> EIMAVDIYVNPPRVDVFHGTPPAWSSFGNKTIWGGNEWVDDSPTRSDIEKRDKEITAYKNTLSAQQKENENKRTEAGKRLSAAIAAREKDENTLKTLRAGNADAADITRQEFRLLQAELREYGFRTEIAGYDALRLHTESRMLFADADSLRISPREARSLIEQAEKRQKDAQNADKKAADML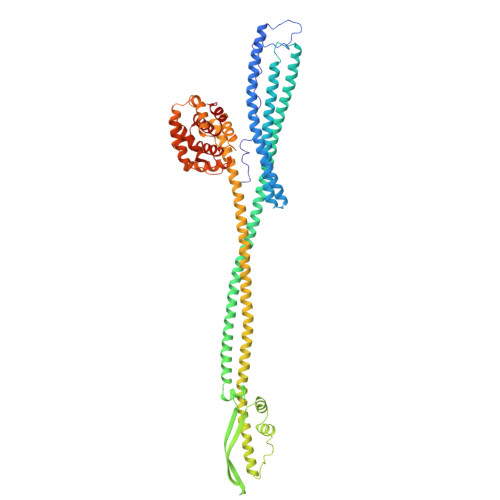AEYERRKGILDTRLSELEKNGGAALAVLDAQQARLLGQQTRNDRAISEARNKLSSVTESLNTARNALTRAEQQLTQQKNTPDGKTIVSPEKFPGRSSTNDSIVVSGDPRFAGTIKITTSAVIDNRANLNYLLSHSGLDYKRNILNDRNPVVTEDVEGDKKIYNAEVAEWDKLRQRLLDARNKITSAESAVNSARNNLSARTNEQKHANDALNALLKEKENIRNQLSGINQKIAEEKRKQDELKATKDAINFTTEFLKSVSEKYGAKAEQLAREMAGQAKGKKIRNVEEALKTYEKYRADINKKINAKDRAAIAAALESVKLSDISSNLNRFSRGLGYAGKFTSLADWITEFGKAVRTENWRPLFVKTETIIAGNAATALVALVFSILTGSALGIIGYGLLMAVTGALIDESLVEKANKFW>HSLLPVDDAINGLSEEQRQLRQTMAKFLQEHLAPKAQEIDRSNEFKNLREFWKQLGNLGVLGITAPVQYGGSGLGYLEHVLVMEEISRASGAVGLSYGAHSNLCINQLVRNGNEAQKEKYLPKLISGEYIGALAMSEPNAGSDVVSMKLKAEKKGNHYILNGNKFWITNGPDADVLIVYAKTDLAAVPASRGITAFIVEKGMPGFSTSKKLDKLGMRGSNTCELIFEDCKIPAANILGHENKGVYVLMSGLDLERLVLAGGPLGLMQAVLDHTIPYLHVREAFGQKIGHFQLMQGKMADMYTRLMACRQYVYNVAK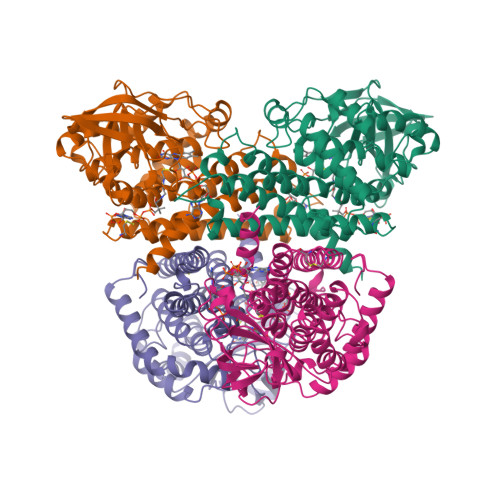ACDEGHCTAKDCAGVILYSAECATQVALDGIQCFGGNGYINDFPMGRFLRDAKLYEIGAGTSEVRRLVIGRAFNADFH[4x]>[2x]ADISLHHRAVLGSTMAYRETGRSDAPHVLFLHGNPTSSYIWRNIMPLVAPVGHCIAPDLIGYGQSGKPDISYRFFDQADYLDALIDELGIASAYLVAQDWGT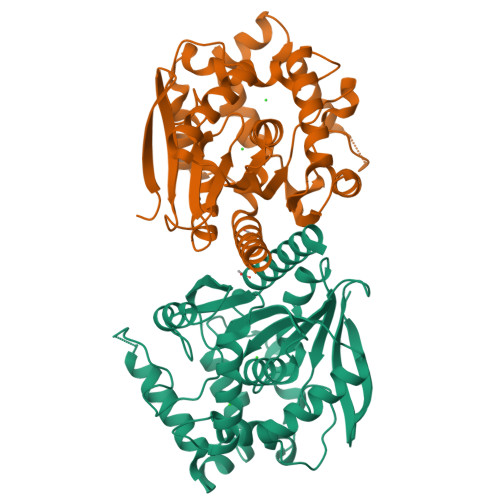ALAFHLAARRPQLVRGLAFMEFIRPMRDWSDFHQHDVAEEQDHAEAARETFRKFRTPGVGEAMILDNNAFVERVLPGSILRTLSEEEMAAYRAPFATRESRMPTLMLPRELPIAGEPADVTQALTAAHAALAASTYPKLLFVGSPGALVSPAFAAEFAKTLKHCAVIQLGAGGHYLQEDHPEAIGRSVAGWIAGIEAASAQRHAALE> AYIGPY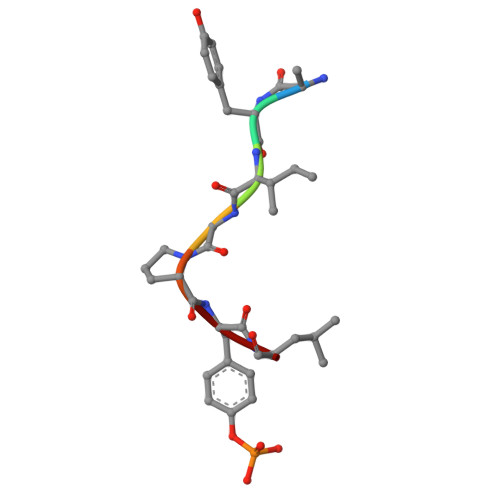L> HVFIRTELSFIKNNVPCIRDMFFIYKRELYNICLDDLKGEEDETHIYVQKKVKDSWITLNDLFKETDLTGRPHIFAYVDVEEIIILLCEDDEFSNRKKDMTCHRFYSNDGKEYQNSEIT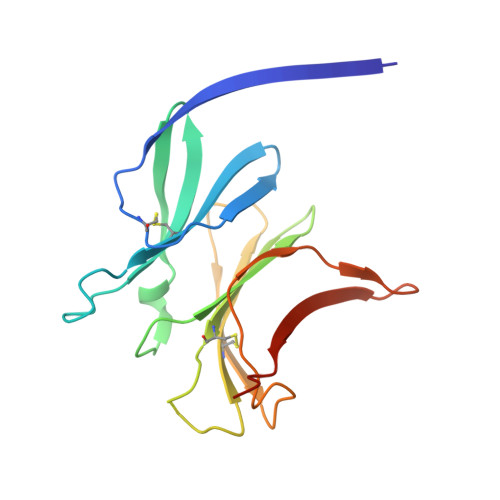ISDYILKDKLLSSYVSLPLKIENREYFLICGVSPYKFKDDNK>MIRRGDVYLADLSPVQGSEQGGVRPVVIIQNDTGNKYSPTVIVAAITGRINKAKIPTHVEIEKKKYKLDKDSVILLEQIRTLDKKRLKEKLTYLSD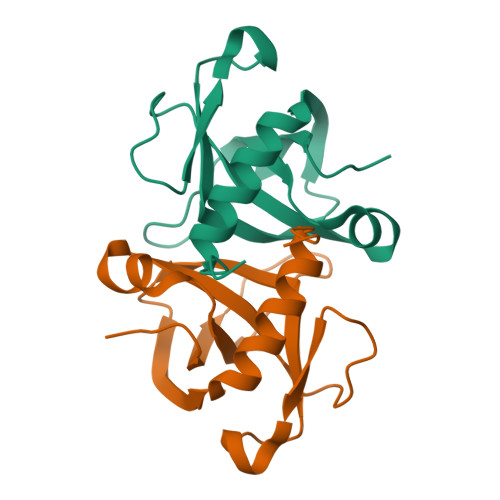DKMKEVDNALMISLGLNAVAHQKNLEHHHHHH[2x]> MKDILEKLEERRAQARLGGGEKRLEAQHKRGKLTARERIELLLDHGSFEEFDMFVQHRSTDFGMEKQKIPGDGVVTGWGTVNGRTVFLFSKDFTVFGGSLSEAHAAKIVKVQDMALKMRAPIIGIFDAGGARIQEGVAALGGYGEVFRRNVAASGVIPQISVIMGPCAGGDVYSPAMTDFIFMVRDTSYMFVTGPDVVKTVTNEVV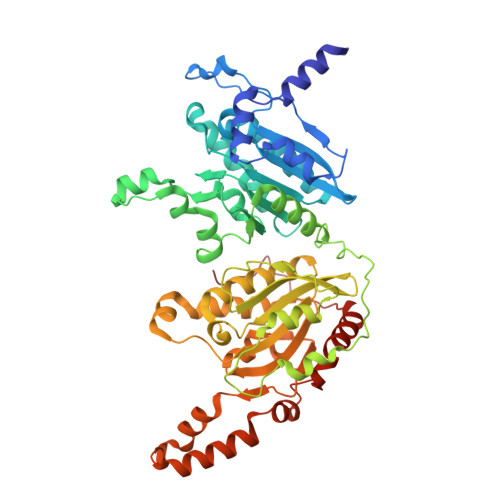TAEELGGAKVHTSKSSIADGSFENDVEAILQIRRLLDFLPANNIEGVPEIESFDDVNRLDKSLDTLIPDNPNKPYDMGELIRRVVDEGDFFEIQAAYARNIITGFGRVEGRTVGFVANQPLVLAGVLDSDASRKAARFVRFCNAFSIPIVTFVDVPGFLPGTAQEYGGLIKHGAKLLFAYSQATVPLVTIITRKAFGGAYDVMASKHVGADLNYAWPTAQIAVMGAKGAVEIIFRAEIGDADKIAERTKEYEDRFLSPFVAAERGYIDEVIMPHSTRKRIARALGMLRTKEMEQPWKKHDNIPL As a well-known tumor suppressor, the tuberous sclerosis complex (TSC) integrates cues of growth factors, energy status, and various stress to maintain Ras homolog enriched in brain (Rheb) in GDP-bound state, and therefore keeps mTORC1 in check to limit undesirable cell growth. The TSC complex acts as a GTPase-activating protein (GAP) toward a small G-protein Rheb required for mTORC1 activation. Mutations of TSC1 or TSC2 genes cause tuberous sclerosis, an autosomal dominant genetic disease characterized by the development of histologically diverse hamartomas or benign tumors, including skin, brain, and kidneys. Here we present the first cryo-EM structure of human TSC complex and elaborate on its characteristic assembly and GAP function.

The structure was determined by cryo-EM single particle reconstruction, and the cryo-EM map was refined to an overall resolution of 4.4 Å. The TSC complex consists of a central core and two wings (termed wing-a and wing-b) and the overall structure exhibits an elongated arch-shaped fold with approximate dimensions of ~390 × 133 × 88 Å3. TSC1, TSC2, and TBC1D7 assemble the TSC complex with a 2:2:1 stoichiometry, generating an asymmetric modular organization. The two TSC2 molecules form a pseudo-symmetric dimer through tail-to-tail interactions. The coiled-coil domains (CCs, residues 746–971) of TSC1a and TSC1b interwind in parallel and form an extended two-helix bundle with the dimer interface being as much as 2386 Å2. The TSC1 dimer makes multiple contacts with TSC2 dimer and stabilizes the overall conformation of the complex. This parallel dimerization of TSC1 leads to an asymmetric formation of TSC1–TSC2 tetramer and recruitment of a single TBC1D7 molecule, generating a unique and characteristic modular organization. Each TSC2 consists of a HEAT repeat domain (HEAT), a dimerization domain (DD), followed by a C-terminal GAP catalytic domain (GAP). The cHEAT–DD–GAP of the two TSC2 molecules adopt pseudo-symmetric fold, whereas the two wHEAT domains adopt distinct conformations due to differently associated TSC1. The TBC1D7 associates with and stabilizes the C-terminal helices (residues 937–971) of TSC1a/1b but has no direct contact with TSC2. The result is consistent with structural observation and supports the notion that TSC2 uses the asparagine thumb (N1643) to accelerate GTP hydrolysis of Rheb and residues K1638, H1640, and L1641 of the catalytic helix function in supporting the conformation of the asparagine thumb.

>MECGLNNRIRMIGQICEVAKTKKFEEHAVEALWKAVADLLQPERPLEARHAVLALLKAIVQGQGERLGVLRALFFKVIKDYPSNEDLHERLEVFKALTDNGRHITYLEEELADFVLQWMDVGLSSEFLLVLVNLVKFNSCYLDEYIARMVQMICLLCVRTASSVDIEVSLQVLDAVVCYNCLPAESLPLFIVTLCRTINVKELCEPCWKLMRNLLGTHLGHSAIYNMCHLMEDRAYMEDAPLLRGAVFFVGMALWGAHRLYSLRNSPTSVLPSFYQAMACPNEVVSYEIVLSITRLIKKYRKELQVVAWDILLNIIERLLQQLQTLDSPELRTIVHDLLTTVEELCDQNEFHGSQERYFELVERCADQRPESSLLNLISYRAQSIHPAKDGWIQNLQALMERFFRSESRGAVRIKVLDVLSFVLLINRQFYEEELINSVVISQLSHIPEDKDHQVRKLATQLLVDLAEGCHTHHFNSLLDIIEKVMARSLSPPPELEERDVAAYSASLEDVKTAVLGLLVILQTKLYTLPASHATRVYEMLVSHIQLHYKHSYTLPIASSIRLQAFDFLLLLRADSLHRLGLPNKDGVVRFSPYCVCDYMEPERGSEKKTSGPLSPPTGPPGPAPAGPAVRLGSVPYSLLFRVLLQCLKQESDWKVLKLVLGRLPESLRYKVLIFTSPCSVDQLCSALCSMLSGPKTLERLRGAPEGFSRTDLHLAVVPVLTALISYHNYLDKTKQREMVYCLEQGLIHRCASQCVVALSICSVEMPDIIIKALPVLVVKLTHISATASMAVPLLEFLSTLARLPHLYRNFAAEQYASVFAISLPYTNPSKFNQYIVCLAHHVIAMWFIRCRLPFRKDFVPFITKGLRSNVLLSFDDTPEKDSFRARSTSLNERPKSRIQTSLTSASLGSADENSVAQADDSLKNLHLELTETCLDMMARYVFSNFTAVPKRSPVGEFLLAGGRTKTWLVGNKLVTVTTSVGTGTRSLLGLDSGELQSGPESSSSPGVHVRQTKEAPAKLESQAGQQVSRGARDRVRSMSGGHGLRVGALDVPASQFLGSATSPGPRTAPAAKPEKASAGTRVPVQEKTNLAAYVPLLTQGWAEILVRRPTGNTSWLMSLENPLSPFSSDINNMPLQELSNALMAAERFKEHRDTALYKSLSVPAASTAKPPPLPRSNTDSAVVMEEGSPGEVPVLVEPPGLEDVEAALGMDRRTDAYSRSSSVSSQEEKSLHAEELVGRGIPIERVVSSEGGRPSVDLSFQPSQPLSKSSSSPELQTLQDILGDPGDKADVGRLSPEVKARSQSGTLDGESAAWSASGEDSRGQPEGPLPSSSPRSPSGLRPRGYTISDSAPSRRGKRVERDALKSRATASNAEKVPGINPSFVFLQLYHSPFFGDESNKPILLPNESQSFERSVQLLDQIPSYDTHKIAVLYVGEGQSNSELAILSNEHGSYRYTEFLTGLGRLIELKDCQPDKVYLGGLDVCGEDGQFTYCWHDDIMQAVFHIATLMPTKDVDKHRCDKKRHLGNDFVSIVYNDSGEDFKLGTIKGQFNFVHVIVTPLDYECNLVSLQCRKDMEGLVDTSVAKIVSDRNLPFVARQMALHANMASQVHHSRSNPTDIYPSKWIARLRHIKRLRQRICEEAAYSNPSLPLVHPPSHSKAPAQTPAEPTPGYEVGQRKRLISSVEDFTEFV[2x];>[2x]MAQQANVGELLAMLDSPMLGVRDDVTAVFKENLNSDRGPMLVNTLVDYYLETSSQPALHILTTLQEPHDKHLLDRINEYVGKAATRLSILSLLGHVIRLQPSWKHKLSQAPLLPSLLKCLKMDTDVVVLTTGVLVLITMLPMIPQSGKQHLLDFFDIFGRLSSWCLKKPGHVAEVYLVHLHASVYALFHRLYGMYPCNFVSFLRSHYSMKENLETFEEVVKPMMEHVRIHPELVTGSKDHELDPRRWKRLETHDVVIECAKISLDPTEASYEDGYSVSHQISARFPHRSADVTTSPYADTQNSYGCATSTPYSTSRLMLLNMPGQLPQTLSSPSTRLITEPPQATLWSPSMVCGMTTPPTSPGNVPPDLSHPYSKVFGTTAGGKGTPLGTPATSPPPAPLCHSDDYVHISLPQATVTPPRKEERMDSARPCLHRQHHLLNDRGSEEPPGSKGSVTLSDLPGFLGDLASEEDSIEKDKEEAAISRELSEITTAEAEPVVPRGGFDSPFYRDSLPGSQRKTHSAASSSQGASVNPEPLHSSLDKLGPDTPKQAFTPIDLPCGSADESPAGDRECQTSLETSIFTPSPCKIPPPTRVGFGSGQPPPYDHLFEVALPKTAHHFVIRKTEELLKKAKGNTEEDGVPSTSPMEVLDRLIQQGADAHSKELNKLPLPSKSVDWTHFGGSPPSDEIRTLRDQLLLLHNQLLYERFKRQQHALRNRRLLRKVIKAAALEEHNAAMKDQLKLQEKDIQMWKVSLQKEQARYNQLQEQRDTMVTKLHSQIRQLQHDREEFYNQSQELQTKLEDCRNMIAELRIELKKANNKVCHTELLLSQVSQKLSNSESVQQQMEFLNRQLLVLGEVNELYLEQLQNKHSDTTKEVEMMKAAYRKELEKNRSHVLQQTQRLDTSQKRILELESHLAKKDHLLLEQKKYLEDVKLQARGQLQAAESRYEAQKRITQVFELEILDLYGRLEKDGLLKKLEEEKAEAAEAAEERLDCCNDGCSDSMVGHNEEASGHNGETKTPRPSSARGSSGSRGGGGSSSSSSELSTPEKPPHQRAGPFSSRWETTMGEASASIPTTVGSLPSSKSFLGMKARELFRNKSESQCDEDGMTSSLSESLKTELGKDLGVEAKIPLNLDGPHPSPPTPDSVGQLHIMDYNETHHEHS;> GVEEKKSLEILLKDDRLDTEKLCTFSQRFPLPSMYRALVWKVLLGILPPHHESHAKVMMYRKEQYLDVLHALKVVRFVSDATPQAEVYLRMYQLESGKLPRSPSFPLEPDDEVFLAIAKAMEEMVEDSVDCYWITRRFVNQLNTKYRDSLPQLPKAFEQYLNLEDGRLLTHLRMCSAAPKLPYDLWFKRCFAGCLPESSLQRVWDKVVSGSCKILVFVAVEILLTFKIKVMALNSAEKITKFLENIPQDSSDAIVSKAIDLWHKHCG> VRELLP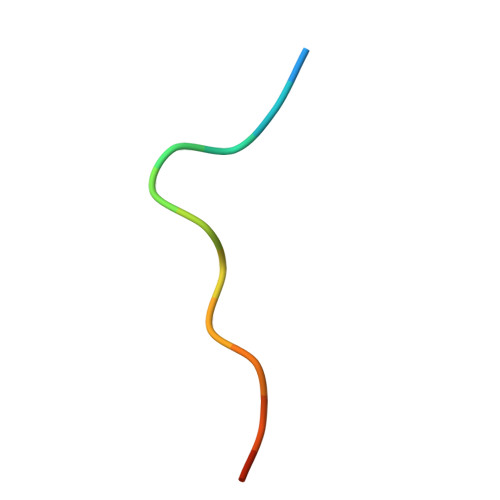ELPHPPSE>[2x]MEKDGLCRADQQYECVAEIGEGAYGKVFKARDLKNGGRFVALKRVRVQTGEEGMPLSTIREVAVLRHLETFEHPNVVRLFDVCTVSRTDRETKLTLVFEHVDQDLTTYLDKVPEPGVPTETIKDMMFQLLRGLDFLHSHRVVHRDLKPQNILVTSSGQIKLADFGLARIYSFQMALTSVVVTLWYRAPEVLLQSSYATPVDLWSVGCIFAEMFRRKPLFRGSSDVDQLGKILDVIGLPGEEDWPRDVALPRQAFHSKSAQPIEKFVTDIDELGKDLLLKCLTFNPAKRISAYSALSHPYFQDLERCKENLDSHLPPSQNTSELNTA;>MAEPWGNELASAAARGDLEQLTSLLQNNVNVNAQNGFGRTALQVMKLGNPEIARRLLLRGANPD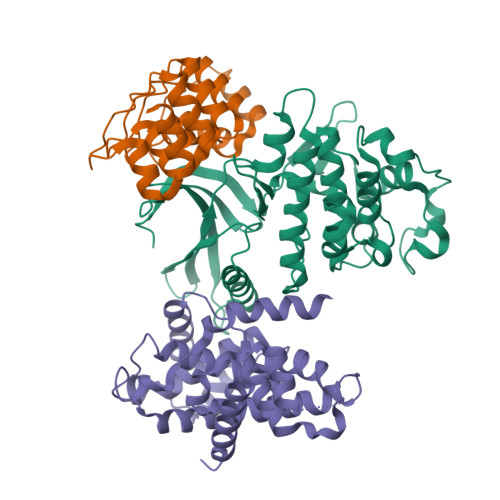LKDRTGFAVIHDAARAGFLDTLQTLLEFQADVNIEDNEGNLPLHLAAKEGHLRVVEFLVKHTASNVGHRNHKGDTACDLARLYGRNEVVSLMQANGAGGATNLQ[2x];>MATANNPPSGLLDPTLCEDRIFYNILEIEPRFLTSDSVFGTFQQSLTSHMRKLLGTWMFSVCQEYNLEPNVVALALNLLDRLLLIKQVSKEHFQKTGSACLLVASKLRSLTPISTSSLCYAAADSFSRQELIDQEKELLEKLAWRTEAVLATDVTSFLLLKLVGGSQHLDFWHHEVNTLITKALVDPLTGSLPASIISAAGCALLVPANVIPQDTHSGGVVPQLASILGCDVSVLQAAVEQILTSVSDFDLRILDSY[2x]>MICSGPQNLAQELKAIGDQLQELQKKLIQGPNISQPRPLLTIETPRHLGEQLNARRKELGIDLYTLELQTGISTSTLKRLFKDPEQVKFGSVFAVANVLGVKLCIGE[2x];>[2x]MHRRVKVLLYGQVV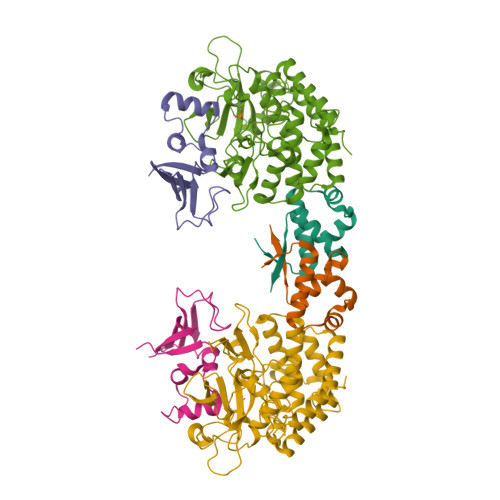GELSQNDSGFLFQYAHDYHGPAISISLPVAQRQFPSETLHPYFASLAPEGWLRQRYSQIQHRDENDLLGMLIDNGKNLLGAIQILPWEE;>[2x]MANCRILLTPLNERDEQRGYSTQGLKRLSGTAKLNPRLGFTRTQFVQELPRQQKGMAISGYQPKLQLVLDEGEFRVVDHQGNFILKPSPADFPGLAENEHATMTLMSRLGFDVPVHGLLSFAPQSEEELEYAFVIRRYDRDNKGLPVHQEQLDGAMQITDKYGKTGNDNEQYVSYETLARFLVAHVNDNIAFKIDLFRRIVYAWLLGNNDMHLRNFGLVYSDGLTPALAPVYDFVSVAPYPEYFYSNYLALPLLTREEGGRELAPGFHSDYGEYIGQDFLLLGESMGLAPRLLEKLFQDIRKENAIVMETYEQSFMTQDHIQAVLQCYRHRLGLLHHHHHH Caudovirales, the taxonomic order for the tailed double-stranded DNA bacteriophages, is characterized by the presence of a tail—a host cell attachment organelle that is connected to the genome-containing spherical or elongated capsid via a neck. We describe cryo-EM structures of the neck, the neck-capsid and neck-tail junctions, and capsid of the Agrobacterium phage Milano. The tail to capsid junction involves a symmetry mismatch that is bridged by the neck, and is therefore crucial for the assembly of tailed phage. The extensive network of disulfide bonds within and between neck, collar, capsid and tail provides an exceptional structural stability to Milano.

The Milano capsid has a T = 9 icosahedral symmetry. It consists of three structural elements that are formed by the MCP (gp9): a pentamer at the icosahedral 5-fold axis, hexamer 1 at the icosahedral 3-fold, and hexamer 2 positioned on a local 2-fold. The icosahedral asymmetric unit is formed by a single subunit of the pentamer, two subunits of hexamer 1, and a complete hexamer 2. Hexamer 1 and hexamer 2 differ in their decorating proteins. The Milano MCP has a HK97-like fold found in all MCPs of dsDNA tailed phages. The conformational plasticity in the P domains, E loops, and N arms of the MCP enable the stable construction of quasi-equivalent pentamers and hexamers. Hexamers and pentamers are further decorated by additional proteins: mCP (gp10) and two linking proteins (LP)—LP1 (gp16) and LP2 (gp128). A dimer of mCP decorates the external surface of the capsid by cementing the pentamer-hexamer 1 and hexamer 1-hexamer 2 interfaces, where it forms disulfide bonds with the MCPs (gp9Cys223—gp10Cys105 and gp9Cys252—gp10Cys74). The resolved parts of LPs—residues 1-13 of LP1 and 1-10 of LP2—occupy quasi-equivalent positions with an mCP at the periphery of pentamer and hexamers and run towards the centers of the pentamers and hexamers, where they interact with the MCPs. Finely, we note that the MCP and mCP are doubly linked: (1) by direct disulfide bonds between MCP and mCP, and (2) through linking proteins LP1 and LP2, which are bound to both MCP and mCP.

>[6x]MDCRNLCGAAAPSRLVQPGCFICRGVAVSIPPAAPGPATSVFDTPPSTFSLRPDGTIIAGTGIRGDHASVGTDGTIEMFIVPFIGDVTGSELTHPYAVELQDGEELAIAFGVTLKSGYGARITEYYDVSLFLENGGNSKELTLQPANTKSGYVWSDGHGYNITDSDGDLHTVQNVTRPVWFEMTEPGIVGVIMEARYKATGLVSSSISITVNVTYAD;>MNFNVGVDFPSFIAWDGEESFPVKVDGFNQFGFTFKTIAALTAATTFNIFYHEPSDADPCVPGPAIRVPEVPFCDTVLLSEDGLAAVTLPETVTPDSFCAGTVPCMNGQWISIAPATGSETNAANVQITVTMKGATR[30x];>[17x]MANKESELNGLDDIHSDIEKLSAHVEKFSDGMDEKYKELTARFDGVKGDNDAIRKAVADATKEYAELSAKHQFFTEELAAMKARLDTPIMRSQAELDDHDRKTAIQLQRNMHEFRGGDPKEFVADESNLVDLKAYRSAVRKMLKVGIESKERVIASMTDVERKAFEASTIGPAFFTPQVLALEVDCNIECASLLDLYGQIEVSRSTFTYMKIADYGQLGEYTCDAKCDAEFGEPGNIRHLEGKTYDYRGVFCFNRKNLQEANYDFLSFMIGAAQRSHRINRNQALMIGKGVNEPKGWLTENCFPVFQTLPVDVNGTSTPAFLAQDWRRFVTSFPAEYGEARSVMHQNVFGYLAAMVDANGRFLFGDGDLTFTPDLVRERIRISNCLPDPTEGNTKGGTGQDAFAAGSFVAAQAAWKTAFYAVEKRPMFFEQYEGGSSAWCVKYQFGAEDGGFVGCCEHGRILQIG;>MVKLNCRPLCQAPTASRLVSPPCFICRGVAPSAPVTPG[11x]>MGDIQVQVNIDDNGKNFDYTYTVTTESELQKVLNELMDYIKKQGAKRVRISITARSSKEAYKFLAILAKVFAELGYNDINRKMTVRFRGDDLEALEKALKEMIRQARKFAGTVTYTLDGNDLEITITGVPRQVLEELAKEAERLAKEFNITITITVTVEGQLGSLEHHHHHH[4x]

Here, we explore the viability of such a mechanism by inserting one de novo designed alpha beta protein into another such that the two beta sheets are combined into one. The backbone geometry at the junctions between the original domains is regularized, and the sequence at the newly formed interface is optimized to stabilize the single integrated domain structure. Crystal structures of two such proteins demonstrate that complex beta sheet structures can be designed with considerable accuracy using this approach and provide a proof-of-concept for the hypothesis that complex beta topologies in natural proteins may have evolved from simpler beta sheet structures in a similar manner. Our success in designing larger beta sheet domains by recombining smaller independently folded beta sheet proteins suggests a similar mechanism could have played a role in the evolution of naturally occurring complex beta sheet proteins.

A first extended sheet protein was created by inserting a designed ferredoxin domain into a beta turn of the designed TOP7 protein to create a half-barrel structure, with the two sheets fused into a single seven strand sheet flanked by four helices. The CD spectra show both alpha and beta structures. The structure shows excellent agreement with the design model, particularly in low B-factor regions, with C-alpha RMSD ranging from 1.76 to 1.85 Å among the four protomers in the crystal. The most similar SCOP domains had weak TM-align scores (0.54 and 0.51), and the sheets in these matched structures have different connectivities than those of the designs, suggesting that the two designed proteins have novel folds. The beta strand connectivity is quite different in the designs than in these closest structural matches.> SMQFSKMHGLGNDFMVVDAVTQNVFFSPELIRRLADAHLGVGFDQLLVVEPPYDPELDFHYRIFNADGSEVAQCGNGARCFARFVRLKGLTNKRDIRVSTANGRMVLTVTDDDLVRVNMGEPNFEPSAVPFRANKAEKTYIMRAAEQTILCGVVSMGNPHCVIQVDDVDTAAVETLGPVLESHERFPERANIGFMQV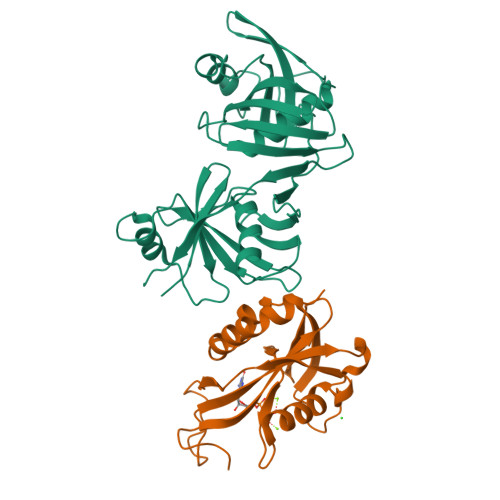VKREHIRLRVYERGAGETQACGSGACAAVAVGIQQGLLAEEVRVELPGGRLDIAWKGPGHPLYMTGPAVHVADGFIHL;> SMIDDDGYRPNVGIVICNRQGQVMWARRFGQHSWQFPQGGINPGESAEQAMYRELFEEVGLSRKDVRILASTRNWLRYKLPKRLVRWDTKPVCIGQKQKWFLLQLVSGDAEINMQTSSTPEFDGWRWVSYWYPVRQVVSFKRDVYRRVMKEFASVVMSLAA> MAGLPRRIIKETQRLLAEPVPGIKAEPDESNARYFHVVIAGPQDSPFEGGTFKLELFLPEEYPMAAPKVRFMTKIYHPNVDKLGRICLDILKDKWSPALQIRTVLLSIQALLSAPNPDDPLANDV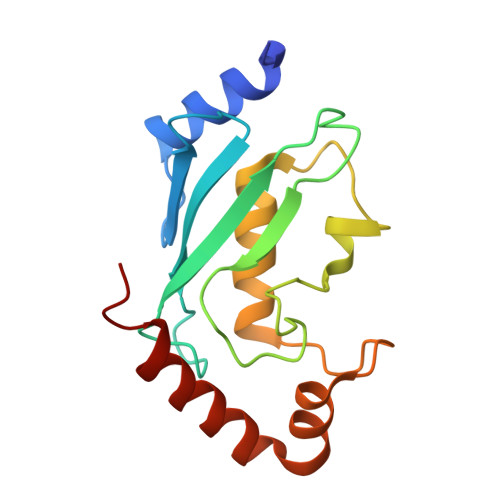AEQWKTNEAQAIETARAWTRLYAMNNI> MGFVNKQFNYKDPVNGVDIAYIKIPNAGQMQPVKAFKIHNKIWVIPERDTFTNPEEGDLNPPPEAKQVPVSYYDSTYLSTDNEKDNYLKGVTKLFERIYSTDLGRMLLTSIVRGIPFWGGSTIDTELKVIDTNCINVIQPDGSYRSEELNLVIIGPSADIIQFECKSFGHEVLNLTRNGYGSTQYIRFSPDFTFGFEESLEVDTNPLLGAGKFATDPAVTLAH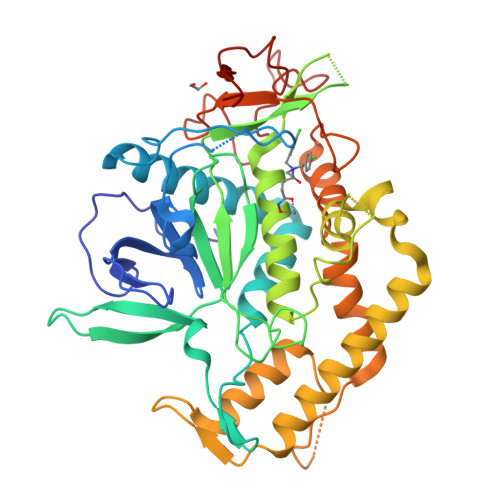ELIHAGHRLYGIAINPNRVFKVNTNAYYEMSGLEVSFEELRTFGGHDAKFIDSLQENEFRLYYYNKFKDIASTLNKAKSIVGTTASLQYMKNVFKEKYLLSEDTSGKFSVDKLKFDKLYKMLTEIYTEDNFVKFFKVLNRKTYLNFDKAVFKINIVPKVNYTIYDGFNLRNTNLAANFNGQNTEINNMNFTKLKNFTGLFEHHHHHH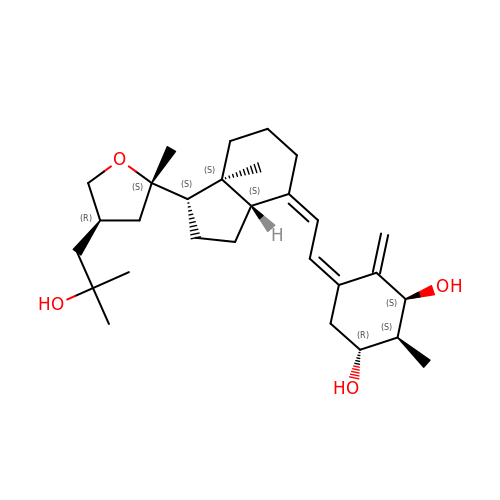(1S,2S,3R,5Z,7E,14beta,17alpha,23R)-23-(2-hydroxy-2-methylpropyl)-2-methyl-20,24-epoxy-9,10-secochola-5,7,10-triene-1,3-diol | C29 H46 O4 | CDTXSCLKUNDXBZ-MWPSFRNWSA-N>MQTEHVILLNAQGVPTGTLEKYAAHTADTRLHLAFSSWLFNAKGQLLVTRRALSKKAWPGVWTNSVCGHPQLGESNEDAVIRRCRYELGVEITPPE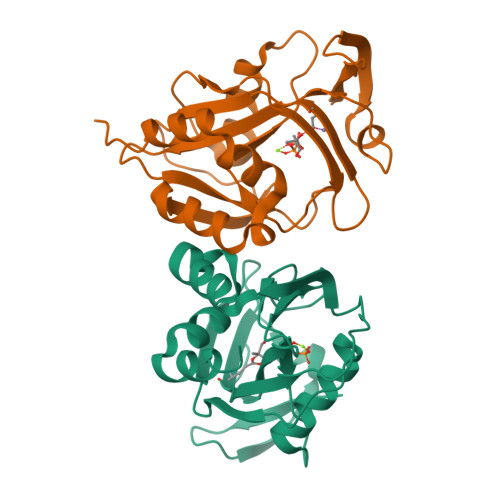SIYPDFRFRATDPSGIVENEVCPVFAARTTSALQINDDEVMDYQWCDLADVLHGIDATPWAFSPWMVMQATNREARKRLSAFTQLKL[2x]7-(5-hydroxy-2-methylphenyl)-8-(2-methoxyphenyl)-1-methyl-1H-imidazo[2,1-f]purine-2,4(3H,8H)-dione | C22 H19 N5 O4 | 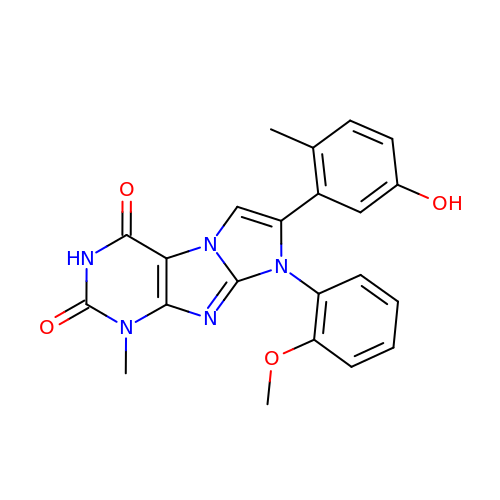JTWMOWRMSZZHDR-UHFFFAOYSA-N DBP is a member of the erythrocyte binding-like (EBL) family of proteins, which localize to micronemes and use Duffy binding-like (DBL) domains to bind specific RBC receptors with high affinity. DBL domains are located in “region II” of EBL proteins, and DBP region II (DBP-RII) is required for formation of a tight junction between Plasmodium and RBC membranes. Two crystal forms were observed, a heterotrimeric complex in which one DARC molecule binds the DBP-RII dimer, and a heterotetrameric complex containing two DARC molecules bound to the DBP-RII dimer.

In the second structure, two DBP-RIIs each bind two DARCs (DARC A and DARC B) creating two DARC binding sites. This architecture creates a heterotetramer, with a total buried surface area of 3628.6 Å2. The heterotetramer structure has a larger translation along the same interface in the same direction, with a second 12 Å displacement relative to the heterotrimer, and a 23 Å displacement relative to the unbound DBP-RII homodimer interface. The directionality of these transitions is consistent with sequential steps in a stepwise mechanism of receptor binding. In the heterotetramer, DBP1 residues R263-I265 and DBP2 residues F261-D264 contact DARC of the opposing monomer. The heterotetrameric complex shows that the DARC molecules are bound in parallel, resulting in a Plasmodium proximal face and a RBC proximal face of DBP-RII. Because only 30 amino acids, DARC residues G31 to S60, separate the structure from the RBC membrane, the surface of the DBP-RII dimer with DARC Y30 is proximal to the RBC membrane, and the alternate surface faces the Plasmodium membrane. Due to avidity contributions to binding inherent in a two-site mechanism, this heterotetrameric complex may enable the observed tight binding of P. vivax to the RBC membrane. The heterotrimer and heterotetramer could represent DBP-RII binding to a DARC heterodimer or homodimer, respectively. The crystallographic and ITC solution studies presented here support a step-wise binding model in which receptor-induced DBP-RII dimerization facilitates formation of a heterotrimer that subsequently recruits a second DARC molecule to form a heterotetramer.

>[2x]ASNTVMKNCNYKRKRRERDWDCNTKKDVCIPDRRYQLCMKELTNLVNNTDTNFHRDITFRKLYLKRKLIYDAAVEGDLLLKLNNYRYNKDFCKDIRWSLGDFGDIIMGTDMEGIGYSKVVENNLRSIFGTDEKAQQRRKQWWNESKAQIWTAMMYSVKKRLKGNFIWICKLNVAVNIEPQIYRWIREWGRDYVSELPTEVQKLKEKCDGKINYTDKKVCKVPPCQNACKSYDQWITRKKNQWDVLSNKFISVKNAEKVQTAGIVTPYDILKQELDEFNEVAFENEINKRDGAYIELCVCSVEEAKKNTQEVVTNVDN;>[2x]GPTGTENSSQLDFEDVWNSSYGVNDSFPDGDYGA> MINEIKKDAQERMDKSVEALKNNLSKVRTGGGGTEERRKDLVKIVRGEAEGGRVAVRNIARDAANDLAALGKDKEVNWFDISQALWEIQK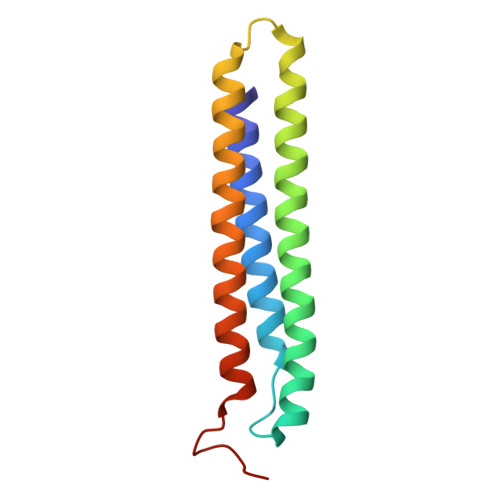LTDVAVKKIDEVLAAKEKELMEVLEHHHHHH> MKVGQDKVVTIRYTLQVEGEVLDQGELSYLHGHRNLIPGLEEALEGREEGEAFQAHVPAEKAYGPHDPEGVQVVPLSAFPEDAEVVPGAQFYAQDMEGNPMPLTVVAVEGEEVTVDFNHPLAGKDLDFQVEVVKVREATPEELLHGHAHPGHHHHHH;>TRYKNAKMLPFAFGA[2x]

Peptidyl-prolyl isomerases (PPIases) catalyze intrinsically slow and often rate-limiting isomerization of prolyl-peptide bonds in unfolded or partially folded proteins, thereby speeding up the folding process and preventing misfolding. An example of such a protein is SlyD (Sensitive to Lysis D), which consists of an FKBP type PPIase domain and a chaperone domain, called IF (insert-in-flap) domain, that has been shown to exhibit chaperone activity. Each of these domains contains one binding site for unfolded proteins or peptides. Often, FKBPs are linked to an additional chaperone domain that can increase their PPIase activity by up to 200-fold.

In order to further explore the contribution of the aromatic residues W4 and F13 of the peptide substrate on the SlyD activity, we changed them individually to negatively charged glutamate (W4E, F13E) or positively charged lysine (W4K, F13K) residues. SlyDWT is less active on peptides with lysine residues in position 4 and 13, similar to the alanine mutants, while the activity towards glutamate variants is increased or unchanged. Similarly, the peptides with positively charged lysine residues at positions 4 (W4K) and 13 (F13K) also displayed only modest changes in their affinities compared to the psWT peptide. Although most of the protein–peptide complexes did not crystallize or yielded crystals of poor diffraction quality, we succeeded in structure determination for four complexes of SlyDWT with bound substrates: psWT, W4A, W4K, and M8A. In all structures, the peptide substrates are bound in the PPIase binding pocket with the proline residue in cis conformation, coordinated by the previously observed protein–peptide polar interactions, namely N35-L9, I37-L9, Y63-F11, H119-F11 and Y92-F13. On the other hand, the conformational flexibility of the residue i − 6 is also reflected in our crystal structures.While residue W4 of the original S2 peptide forms a polar interaction with the SlyD residue E60, orienting the N-terminus of the peptide outside of the binding pocket, mutant peptide residues A4 and K4 do not form this interaction and as a result, the peptide N-terminus bends towards the SlyD linker region. Taken together, while different side chains at position 4 assume distinct conformations in each substrate variant, these conformations proof to be unspecific when compared to the structure of other variants. This resembles encounter complexes where initial contacts are unspecific and contribute to the association reaction, but not to the dissociation step where they are replaced by specific contacts. When both binding sites are fully occupied, the two domains restrict access to the PPIase domain binding site in the tight conformation. Here, the release of the substrate from the FKBP binding site is likely hindered.>NQPDWADEAANGAHQDAWKSLKARVENVYYMVKATYKNDPVWGNDFTCVGVMANDVNEDEKSIQAEFLFMNNADTNMQFATEKVTAVKMYGYNRENAFRYETEDGQVFTDVIAYSD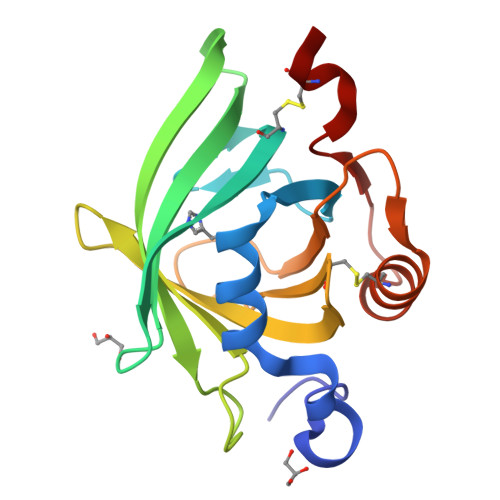DNCDVIYVPGTDGNEEGYELWTTDYDNIPANCLNKFNEYAVGRETRDVFTSACLE[2x]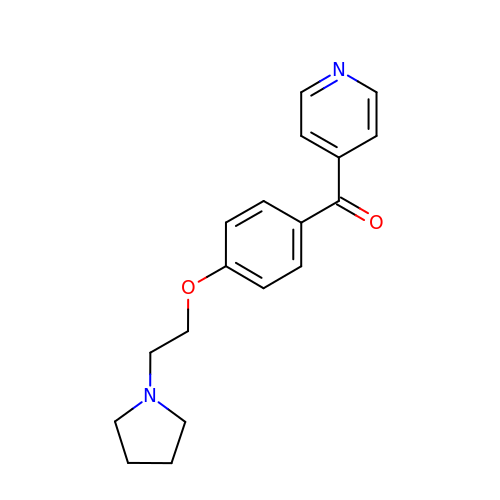pyridin-4-yl[4-(2-pyrrolidin-1-ylethoxy)phenyl]methanone | C18 H20 N2 O2 | AFGONOGEOHNVPG-UHFFFAOYSA-N> MASPPHQQLLQHHSTEVSCDSSGDSNSVRVRINPKQPSSNSHPKHCKYSISSSCSSSGDSGGVPRRMGAGGRLRRRKKLPQLFERASSRWWDPKFDSVNLEEACMERCFPQTQRRFRYALFYIGFACLLWSIYFGVHMKSKLIVMVAPALCFLVVCVGFFLFTFTKLYARHYVWTSLVLTLLVFALTLAAQFQVLTPLSGRVDNFNHTRAARPTDTCLSQVGSFSMCIEVLFLLYTVMHLPLYLSLILGVAYSVLFETFGYHFQDEACFASPGAEALHWELLSRALLHLCIHAIGIHLFIMSQVRSRSTFLKVGQSIMHGKDLEVEKALKERMIHSVMPRIIADDLMKQGDEESENSVKRHATSSPKNRKKKSSIQKAPIAFRPFKMQQIEEVSILFADIVGFTKMSANKSAHALVGLLNDLFGRFDRLCEETKCEKISTLGDCYYCVAGCPEPRADHAYCCIEMGLGMIRAIEQFCQEKKEMVNMRVGVHTGTVLCGILGMRRFKFDVWSNDVNLANLMEQLGVAGKVHISEATAKYLDDRYEMEDGKVTERLGQSVVADQLKGLKTYLIAGQRAKESHCSCSEALLSGFEVLDGSRVSSGPRGQGTASPGSVSDLAQTVKTFDNLKTCPSCGITFTPKPEAGAEGGAVQNGCQEEPKNSAKASGGPSSKTQNGLLSPPPEEKLTNSQTSLCEILQEKGRWAGVSLDQSALLPLRFKNIREKTDAHFVDVIKEDSLMKDYFFKPPINQFSLNFLDPELERAYRTSYQEEVVKSSPVRTFASATFSSLLDVLLSTTVFLILSITCFLRYGAASTPPPPAALAVFGAALLLEILSLVVSVRMVFFLEDVMTCTKRLLEWIAGWLPRHFIGAILVSLPALAVYSHVTSEFETNIHSTMFTGSAVLTAVVQYCNFCQLSSWMRSSLATVVGAGPLLLLLYVSLCPDSSTVISHLDAVQNFSSTRKLCNASLPHDGRSPASLIGQEVILVFFLLLLLVWFLNREFEVSYRLHYHGDVEADLHRTKIQSMRDQADWLLRNIIPYHVAEQLKVSQTYSKNHDSGGVIFASIVNFSEFYEENYEGGKECYRVLNELIGDFDELLSKPDYSSIEKIKTIGATYMAASGLNATQCRDGSHPQEHLQILFEFAKEMMRVVDDFNNNMLWFNFKLRVGFNHGPLTAGVIGTTKLLYDIWGDTVNIASRMDTTGVECRIQVSEESY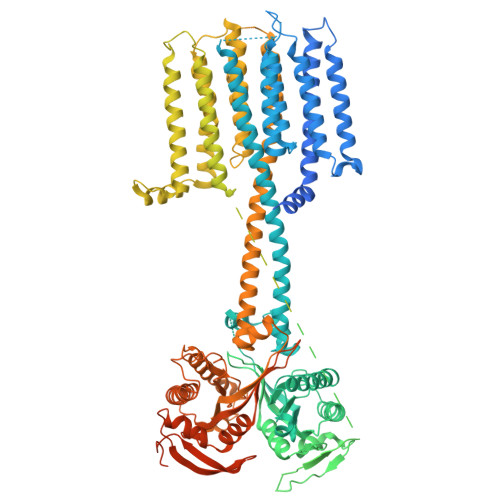RVLSKMGYEFDYRGTVNVKGKGQMKTYLYPKCTDSGLVPQHQLSISPDIRVQVDGSIGRSPTDEIASLVPSVQNPDQVPPGSENNAQTRDAHPSAKRPWKEPVRAEERCRFGKAIEKSDCEEVGMEEANELTKLNVSERA> G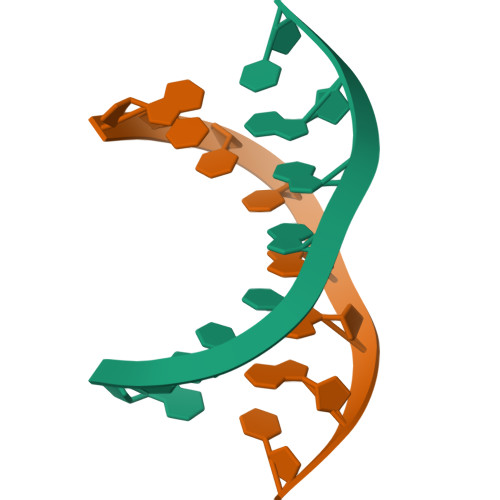CCCGAGC>YVEFVAQISPQYPMFTVPLPIPPVKQPRLTVTNPVNGQEIWYYEVEIKPFTHQVYPDLGSADLVGYDGMSPGPTFQVPRGVETVVRFINNAEAPNSVHLHGSFSRAAFDGWAEDITEPGSFKDYYYPNRQSARTLWYHDHAMHITAENAYRGQAGLYMLTDPAEDALNLPSGYGEFDIPMILTSKQYTANGNLVTTNGELNSFWG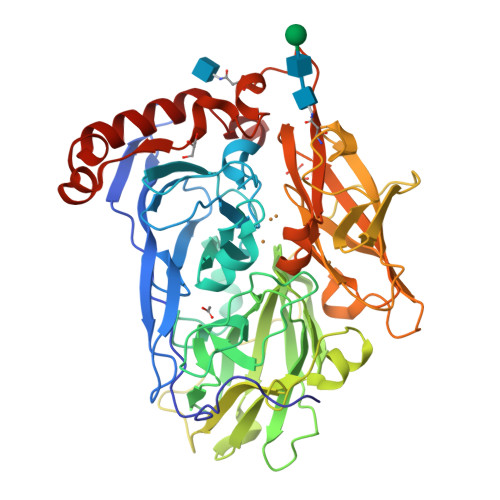DVIHVNGQPWPFKNVEPRKYRFRFLDAAVSRSFGLYFADTDAIDTRLPFKVIASDSGLLEHPADTSLLYISMAERYEVVFDFSDYAGKTIELRNLGGSIGGIGTDTDYDNTDKVMRFVVADDTTQPDTSVVPANLRDVPFPSPTTNTPRQFRFGRTGPTWTINGVAFADVQNRLLANVPVGTVERWELINAGNGWTHPIHIHLVDFKVISRTSGNNARTVMPYESGLKDVVWLGRRETVVVEAHYAPFPGVYMFHCHNLIHEDHDQMAAFNATVLPDYGYNATVFVDPMEELWQARPYELGEFQAQSGQFSVQAVTERIQTMAEYRPYAAADE[2x]>[2x]MSITLSDSAAARVNTFLANRG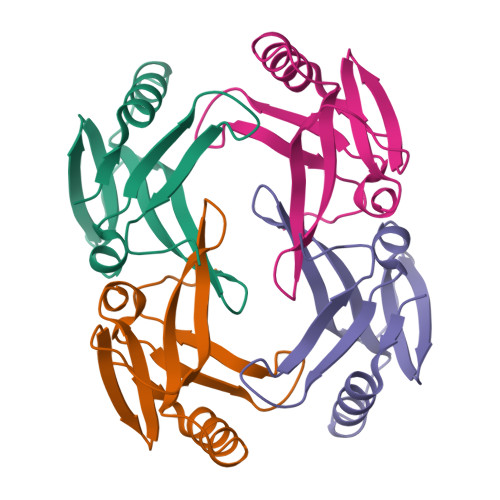KGFGLRLGVRTSGCSGMAYVLEFVDEPTPEDIVFEDKGVKVVVDGKSMQFLDGTQLDFVKEGLNEGFKFTNPNVKDECGCGESFHV>[2x]SYGDNAQNGGGLVIDMPALNRIHSIDSGTRLVDVDAGVSLDQLMKAALPHGLWVPVLPGTRQVTVGGAIGC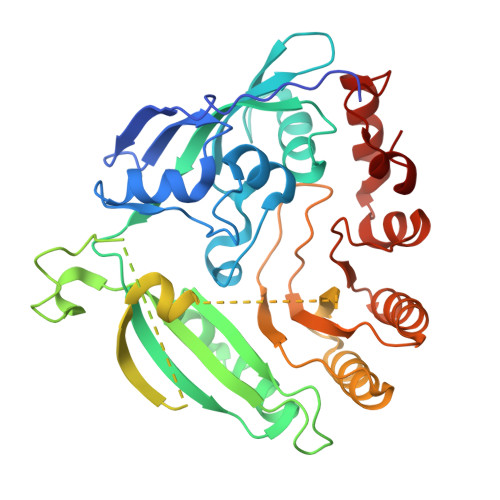DIHGKNHHSAGSFGNHVRSMELLTANGEVRHLTPAGPDSDLFWATVGGNGLTGIILRATIEMTPTETAYFIADGDVTGSLDETIAFHSDGSEANYTYSSAWFDAISKPPKLGRAAISRGSLAKLDQLPSKLQKDPLKFDAPQLLTLPDIFPNGLANKFTFMPIGELWYRKSGTYRNKVQNLTQFYHPLDMFGEWNRAYGSAGFLQYQFVVPTEAVEEFKSIIVDIQRSGHYSFLNVFKLFGPGNQAPLSFPIPGWNVCVDFPIKAGLHEFVTELDRRVLEFGGRLYTAKDSRTTAETFHAMYPRIDEWIRIRRSVDPDGVFASDMARRLQLL>NNPNLDMSGWLMNLKGVVNSKVELEGLSGSDGQVVLMTGYYAGQYMGGDHFKYDSTQALINNGVTVINGWVKQFSAGVLTVSACGADPSASDHSAALDLAVNTATSLKRKLVVDFDLRVNTTTELDATLRIEGDGGAVQFSRSITATADIPIFTVKAGFSSESSYFGKLMFKASTGGTATAFRSTSNGYLSQSTFDHCVFDRSLRYGIDANLILCDFQKCDFGTYMSTTNSIGFKAIRSLGVVGTREPNANTFYNCIFRKGTDDCMIEWDSYGTQWHFFACDLEQNLCTEALIKCTASSPI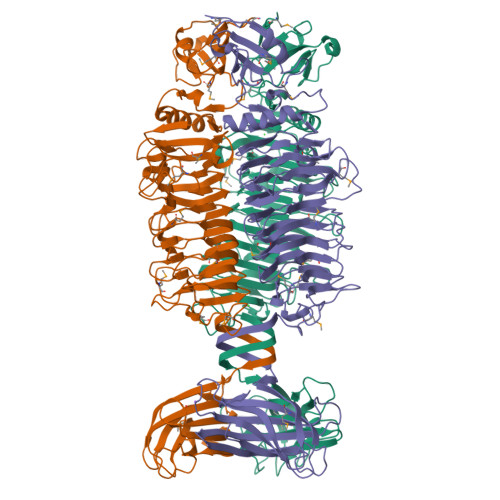MFVGGYIEANTSTPYVIKTLGNSATGFVPLIKFQGIHMNRPCSVAIGKNTMANYPKYIFEGCYGQLISAVVESSTGVLNDVALIENSIANHFTLATGGSIGDIRTLTMPSGFNADSRNFQAAKITNLTSYKHNYKKTINRDFTVGSSVGVASLSHPSISGASYGGRLLVNAIFGTTAAAGTNSAVYELLVTSVGTAKYISQIGSAGLTSGAAASHPSFTWSINSSNVLVATAVGSTAGRFAMEVFTTGNVQAT[6x]3-[(cyclopropylamino)methyl]-8-ethylquinolin-2(1H)-one | C15 H18 N2 O | 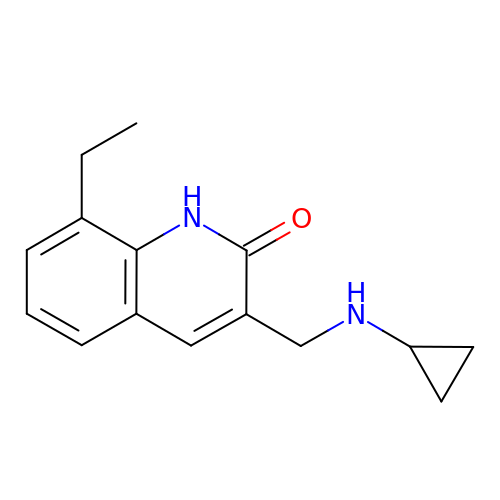NRYCDZCJUHABBD-UHFFFAOYSA-N>[2x]ANSKLTSDFDNPRWIGRHKHMFNFLDVNHNGKISLDEMVYKASDIVINNLGATPE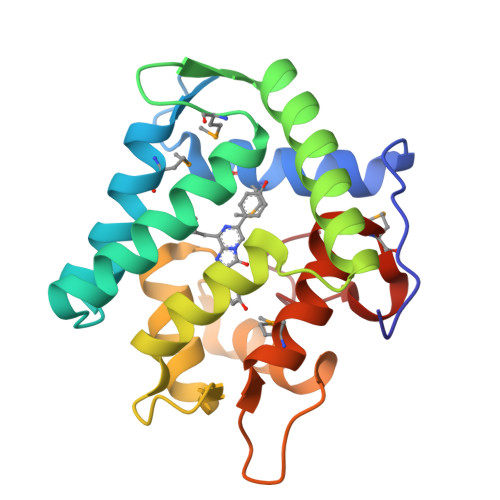QAKRHKDAVEAFFGGAGMKYGVETDWPAYIEGWKKLATDELEKYAKNEPTLIRIWGDALFDIVDKDQNGAITLDEWKAYTKAAGIIQSSEDCEETFRVCDIDESGQLDVDEMTRQHLGFWYTMDPACEKLYGGAVP(2R)-2-hydroxy-N,N,N-trimethyl-2-phosphonoethan-1-aminium | C5 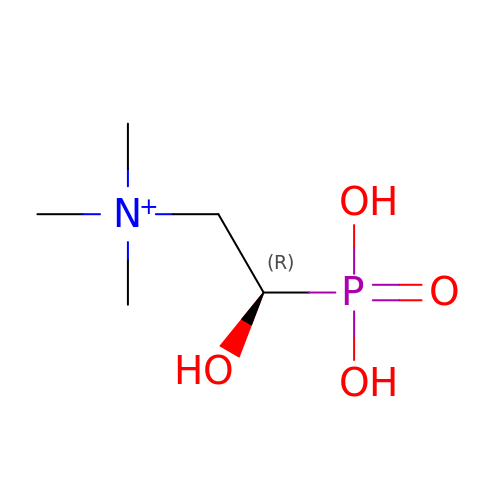H15 N O4 P | YJIOAKRBBHTUPD-RXMQYKEDSA-O Myelin-gene Regulatory Factor (MyRF, also known as MRF, Gm98 or C11Orf9 in human) is considered one of the master transcription factors for myelin production by oligodendrocytes in the central nervous system, which permits action potentials to propagate by saltatory conduction along axons and is very important for powerful brain functions. MyRF was revealed as a transmembrane (TM) protein located at the endoplasmic reticulum (ER) membrane. Its cytoplasmic portion contains an N-terminal proline-rich region and a following DNA binding domain (DBD) which can be auto-cleaved from the ER membrane by a region between the DNA-binding and TM domains. After cleavage, the N-terminal part of MyRF releases from the ER membrane and enters the cell nucleus guided by the NLS signal within its sequence to activate myelin gene expression.

Using limited proteolysis, we generated a proteolytically resistant DBD core that is about 24kD. The structural model has been completed and refined to 2.46 Å resolution (Rwork = 18% and Rfree = 23%). The space group is P321 (104.0, 104.0, 46.7, 90, 90, 120), with one molecule per asymmetric unit. Of the 210 amino acids corresponding to the DBD, only residues 351–532 were clearly visible in the electron density map. The main part of MyRF DBD consists of two antiparallel β-sheets that have three strands (a, b and e) and five strands (c’, c, f, g and β1) respectively, labeled according to the standard nomenclature of Ig-fold. The sheets pack against each other, forming a β-sandwich with a “Greek key” topology. MyRF DBD forms a trimer with a crystallographic three-fold symmetry axis in the crystal. Residues 438–442 of the loop between strand c and β7 from one protomer form 3 hydrogen bond interactions with residues 469–471 of strand e from the neighboring protomer. Residues 354–360 of the loop between strand β1 and β2 from one protomer form 4 hydrogen bond interactions with residues 371–377 of the loop before strand a from the other protomer. The electrostatic surface potential measurement of MyRF DBD structure reveals a highly electropositive surface owing to the presence of lysine and arginine residues at the bottom of the β-barrel core. In particular, 3 conserved alkaline residues in MyRF (K399, R454 and R478) are superimposable with the residues of Ndt80 (R111, R177 and R254) interacting at the major groove of DNA, implying that they may be involved in interaction with DNA too.

> GPEIIKWQPHQQNKWATLYDANYKELPMLTYRVDADKGFNFSVGDDAFVCQKKNHFQVTVYIGMLGEPKYVKTPEGLKPLDCFYLKLHGVKLEALNQSINIEQSQSDRSKRPFNPVTVNLPPEQVTKVTVGRLHFSETTANNMRKKGKPNPDQRYFMLVVALQAHAQNQNYTLAAQISERIIVRAS> PQRVAAHITGTRGRSNTLSSPNSKNEKALGRKINSWESSRSGHSFLSNLHLRNGELVIHEKGFYYIYSQTYFRFQEEIKENTKNDKQMVQYIYKYTSYPDPILLMKSARNSCWSKDAEYGLYSIYQGGIFELKENDRIFVSV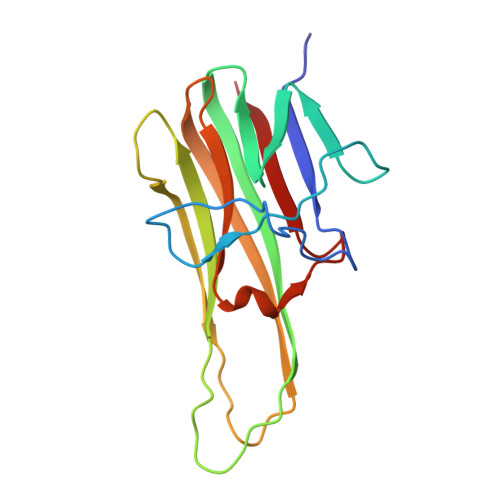TNEHLIDMDHEASFFGAFLVG>APTSSSTKKTQLQLEHLLLDLQMILNGINNYKNPKLTRMLTFKFYMPKKATELKHLQCLEEELKPLEEALNLAQSKNFHLRPRDLISNINVIVLELKGSETTFMCEYADET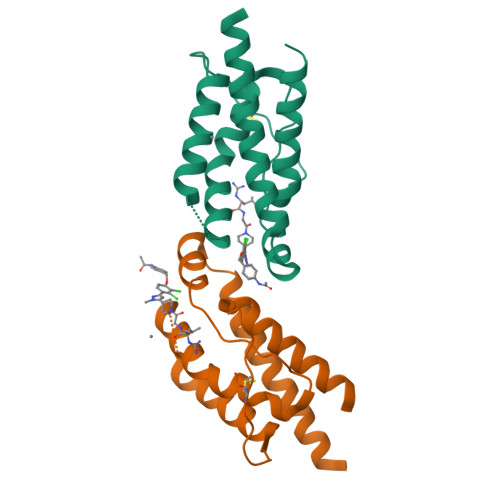ATIVEFLNRWITFCQSIISTL[4x]> MGSSHHHHHHSQDPNSM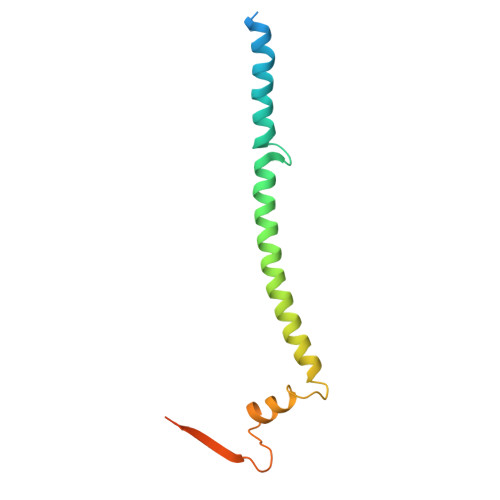GKLTLLLLAILVWLQYSLWFGKNGIHDYTRVNDDVAAQQATNAKLKARNDQLFAEIDHLNGGQEALEERARNELSMTRPGETFYRLVPDASKRAQSAGQNNR> MENKNGTAATTQQSAANMLAAHKGVNQAPVPLKMERVGPHDVHIEMTAQITDIEIDKGKIYKAWTFNGQAPGPLVVVNE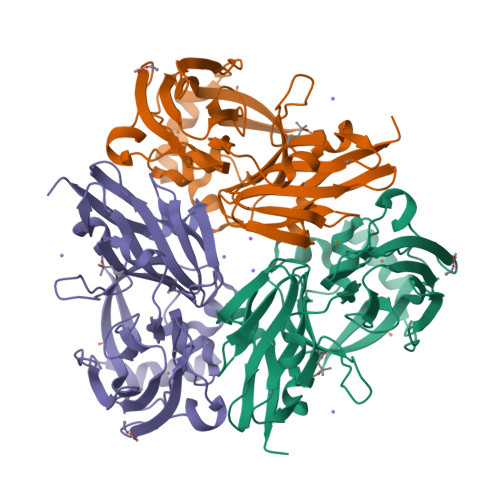GDTIHFTLKNMDPVVPHSMDFHAVHASPSKDFIDVMPNKSGTFTYPANKPGVFMYHCGTKPVLQHIANGMHGVIIVKPKNGYPTDKEVDREYVLIQNEWYKYNDMNDFQNGVPSYVVFSSKALKPGDPNTNGDTFTLKEKPLLAKVGEKIRLYINNVGPNEVSSFHVVGTVFDDVYLDGNPNNHLQGMQTVMLPASGGAVVEFTVTRPGTYPIVTHQFNHAQKGAVAMLKVTETGEDDGSETSGH> IE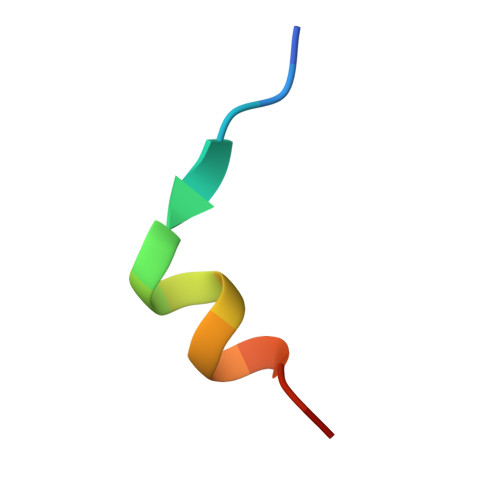VWDYEQLREEYGF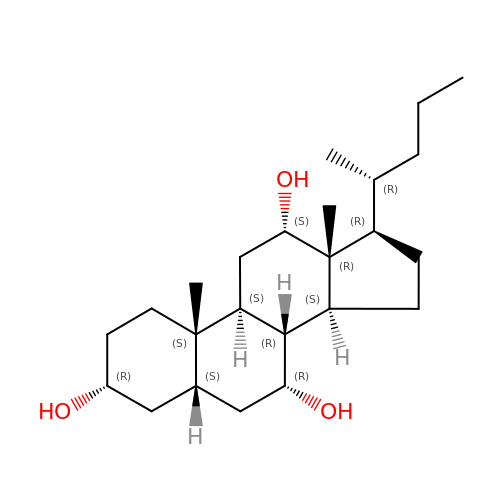(3R,5S,7R,8R,9S,10S,12S,13R,14S,17R)-10,13-dimethyl-17-[(2R)-pentan-2-yl]-2,3,4,5,6,7,8,9,11,12,14,15,16,17-tetradecahydro-1H-cyclopenta[a]phenanthrene-3,7,12-triol | C24 H42 O3 | PFZUIDNKXWIWBG-YHEMGIGTSA-N> GPLGSMTIIESNYISVREEYPDIDSEVRAILLSHAQNGITISSIKSEYRKLTGNPFPLHDNVTDFLLTIPNVT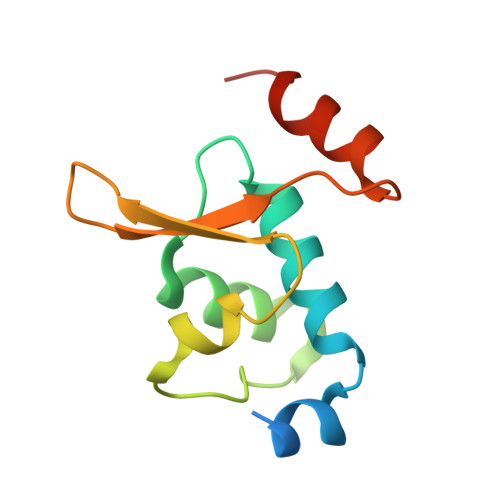AECSESGKRIFNLKASLKNGHLLDMVLNQKERTS>[2x]MTADELVFFVNGKKVVEKNADPETTLLVYLRRKLGLCGTKLGCGEGGCGACTVMISKYDRLQNKIVHFSVNACLAPICSLHHVAVTTVEGIGNTQKLHPVQERIARSHGSQCGFCTPGIVMSMYTLLRNQPEPTVEEIENAFQGNLCRCTGYRPILQGFRTFAKDGGCCGGSGNNPNCCMNQTKDQTVSLSPSLFNPEDFKPLDPTQEPIFPPELLRLKDTPQKKLRFEGERVTWIQASTMEELLDLKAQHPDAKLVVGNTEIGIEMKFKNMLFPLIVCPAWIPELNSVVHGPEGISFGASCPLSLVESVLAEEIAKLPEQKTEVFRGVMEQLRALAGKQVKSVASIGGNIITASPISDLNPVFMASGAKLTLVSRGTRRTVRMDHTFFPGYRKTLLRPEEILLSIEIPYSKEGEFFSAFKQASRREDDIAKVTSGMRVLFKPGTIEVQELSLCFGGMADRTISALKTTPKQLSKSWNEELLQSVCAGLAEELQLAPDAPGGMVEFRRTLTLSFFFKFYLTVLQKLGRADLEDMCGKLDPTFASATLLFQKDPPANVQLFQEVPKDQSEEDMVGRPLPHLAANMQASGEAVYCDDIPRYENELSLRLVTSTRAHAKITSIDTSEAKKVPGFVCFLTAEDVPNSNATGLFNDETVFAKDEVTCVGHIIGAVVADTPEHAQRAARGVKITYEDLPAIITIQDAIN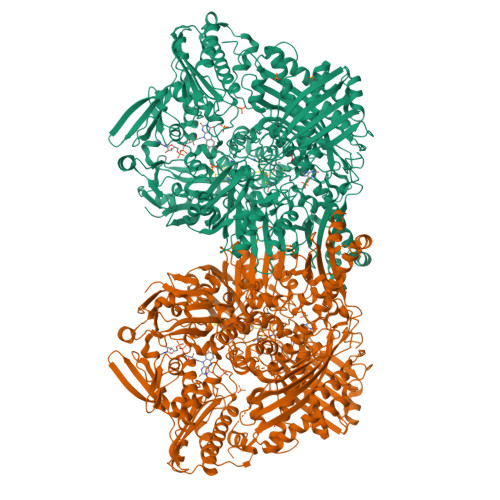NNSFYGSEIKIEKGDLKKGFSEADNVVSGELYIGGQEHFYLETNCTIAVPKGEAGEMELFVSTQNTMKTQSFVAKMLGVPDNRIVVRVKRMGGGFGGKETRSTVVSTALALAAHKTGRPVRCMLDRDEDMLITGGRHPFLAKYKVGFMKTGTVVALEVAHFSNGGNTEDLSRSIMERALFHMDNAYKIPNIRGTGRICKTNLPSNTAFRGFGGPQGMLIAEYWMSEVAITCGLPAEEVRRKNMYKEGDLTHFNQKLEGFTLPRCWDECIASSQYLARKREVEKFNRENCWKKRGLCIIPTKFGISFTLPFLNQGGALVHVYTDGSVLLTHGGTEMGQGLHTKMVQVASRALKIPTSKIHISETSTNTVPNTSPTAASASADLNGQGVYEACQTILKRLEPFKKKKPTGPWEAWVMDAYTSAVSLSATGFYKTPNLGYSFETNSGNPFHYFSYGVACSEVEIDCLTGDHKNLRTDIVMDVGSSLNPAIDIGQVEGAFVQGLGLFTMEELHYSPEGSLHTRGPSTYKIPAFGSIPIEFRVSLLRDCPNKRAIYASKAVGEPPLFLASSIFFAIKDAIRAARAQHGDNAKQLFQLDSPATPEKIRNACVDQFTTLCVTGVPENCKSWSVRI> QRPR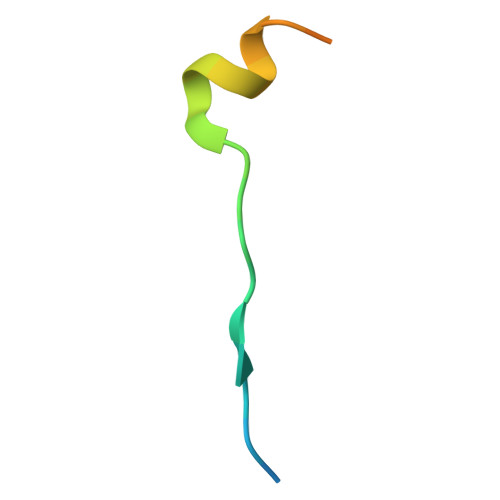PRVLLKAPTLAEMEEMNTSEEEE>GSMAAADEPKPKKLKVEAPQALSENVLFGMGNPLLDISAVVDKDFLDKYSLKPNDQILAEDKHKELFDELVKKFKVEYHAGGSTQNSMKVAQWLIQEPHKAATFFGCIGIDKFGEILKRKAADAHVDAHYYEQNEQPTGTCAACITGGNRSLVANLAAANCYKKEKHLDLERNWVLVEKARVYYIAGFFLTVSPESVLKVARYAAENNRVFTLNLSAPFISQFFKEALMDVMPYVDILFGNETEAATFAREQGFETKDIKEIAKKAQALPKVNSKRQRTVIFTQGR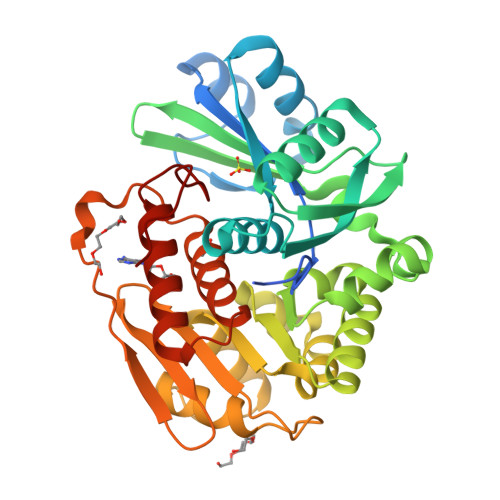DDTIVAAENDVTAFPVLDQNQEEIIDTNGAGDAFVGGFLSQLVSDKPLTECIRAGHYAASVIIRRTGCTFPEKPDFH[2x]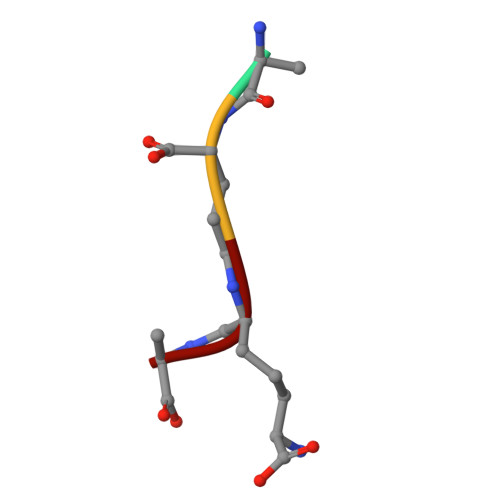> AEKA>[2x]GSHMASPNGQTKPLPALKLALEYIVPAMNK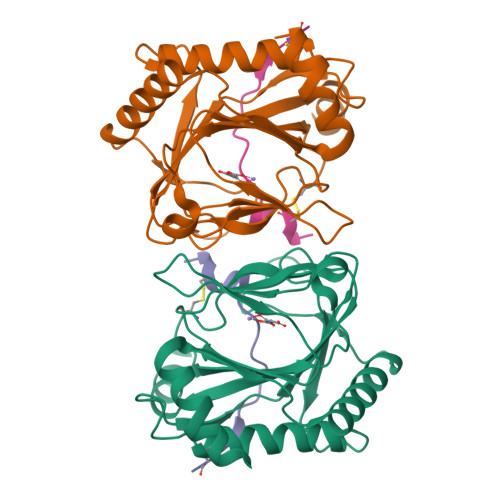HGICVVDDFLGKETGQQIGDEVRALHDTGKFTDGQLVSQKSDSSKDIRGDKITWIEGKEPGCETIGLLMSSMDDLICHCNGKLGSYKINGRTKAMVACYPGNGTGYVRHVDNCNGDGRCVTCIYYLNKDWDAKVSGGILRIFPEGKAQFADIEPKFDRLLFFWSDRRNPHEVQPAYATRYAITVWYFDADETAAAKVKYLTGEKGVRVELNKPSDSVGKDVF;>[2x]DACTLLAPAAGDTIISLCF>[2x]ETGTVPAINYLGAGYDHVRGNPVGDPSSMGDPGIRPPVLRFTYAQNEDGVSNDLTVLQPLGGYVRQYVACRQSETISELSNLSDYQNELSVDASLQGGDPIGLNSFSASTGYRDFAKEVS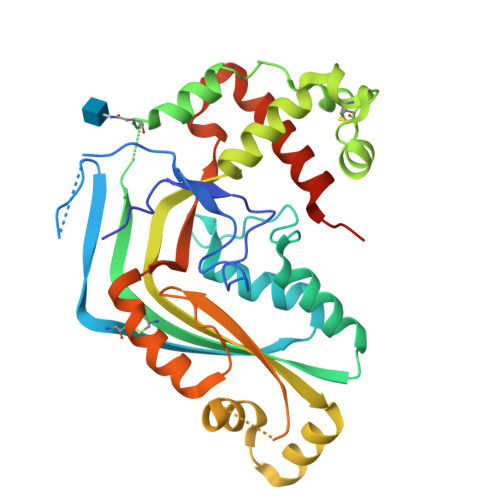KKDTRTYMLKNYCMRYEAGVAQSNHFKWNVTLAFAAGVSQLPDVFDAHNPECACSAEQWRQDQNAEACTKTNVPIWISFIEQFGTHFLVRLFAGGKMTYQVTAKRSEVEKMRNMGIDVKTQLKMQLGGVSGGAGQGTSSKKQQSSSEYQMNVQKETLVIGGRPPGQVSDPAALAAWADTVEELPMPVKFEVQPLYHLLPVEKQEAFKQAVTFYSKAVGLTPQDLSALGTKHHHHHH> MRVWSEVQAAHMATVGQLLGGARKVAKTRKCRIRQLDGSPFKKGICLRVYTTSPKKPNSANRKLAKVQLSNGLKALAYIPGEGHNLQEHSMVLVSG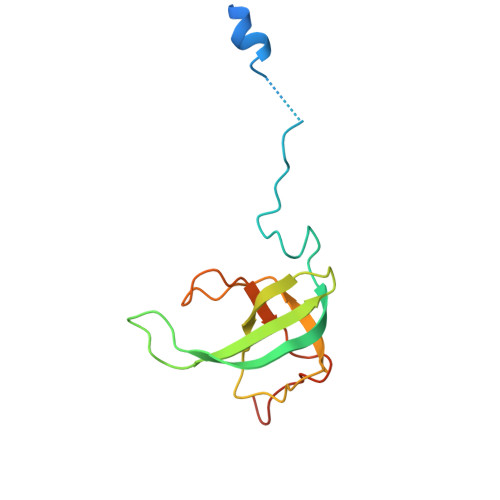NGVRDLPGVKLRIVRGRYDCAGVKDRKKSSED>MKVLVTGFEPFGGEKINPTERIAKDLDGIKIGDAQVFGRVLPVVFGKAKEVLEKTLEEIKPDIAIHVGLAPGRSAISIERIAVNAIDARIPDNEGK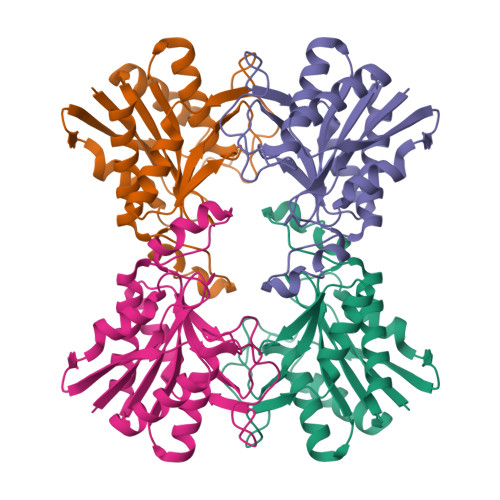KIEDEPIVPGAPTAYFSTLPIKKIMKKLHERGIPAYISNSAGLYLSNYVMYLSLHHSATKGYPKMSGFIHVPYIPEQIIDKIGKGQVPPSMSYEMVLEAVKVAIEVALEELL[4x]>MDYKDDDDKGEDGKPVWAPHPTDGFQVGNIVDIGPDSLTIEPLNQKGKTFLALINQVFPAEEDSKKDVEDNCSLMYLNEATLLHNIKVRYSKDRIYTYVANILIAVNPYFDIPKIYSSETIKSYQGKSLGTMPPHVFAIADKAFRDMKVLKLSQSIIVSGESGAGKTENTKFVLRYLTESYGTG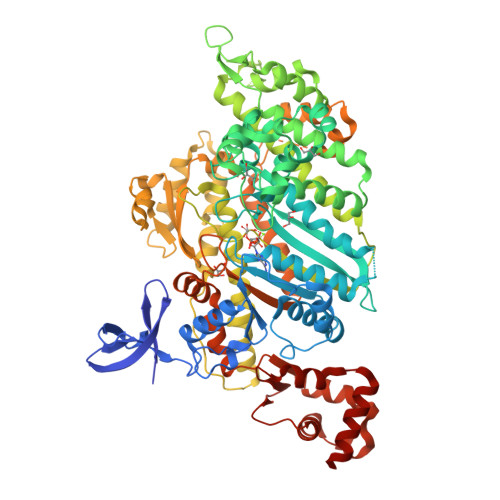QDIDDRIVEANPLLEAFGNAKTVRNNNSSRFGKFVEIHFNEKSSVVGGFVSHYLLEKSRICVQGKEERNYHIFYRLCAGASEDIRERLHLSSPDNFRYLNRGCTRYFANKETDKQILQNRKSPEYLKAGSLKDPLLDDHGDFIRMCTAMKKIGLDDEEKLDLFRVVAGVLHLGNIDFEEAGSTSGGCNLKNKSTQALEYCAELLGLDQDDLRVSLTTRVMLTTAGGAKGTVIKVPLKVEQANNARDALAKTVYSHLFDHVVNRVNQCFPFETSSYFIGVLDIAGFEYFEHNSFEQFCINYCNEKLQQFFNERILKEEQELYQKEGLGVNEVHYVDNQDCIDLIEARLVGILDILDEENRLPQPSDQHFTSAVHQKHKDHFRLSIPRKSKLAIHRNIRDDEGFIIRHFAGAVCYETTQFVEKNNDALHMSLESLICESRDKFIRELFESSTNNNKDTKQKAGKLSFISVGNKFKTQLNLLLDKLRSTGASFIRCIKPNLKMTSHHFEGAQILSQLQCSGMVSVLDLMQGGFPSRASFHELYNMYKKYMPDKLARLDPRLFCKALFKALGLNEIDYKFGLTKVFFRPGKFAEFDQIMKSDPDHLAELVKRVNHWLI[2x]>[4x]MAIHNPL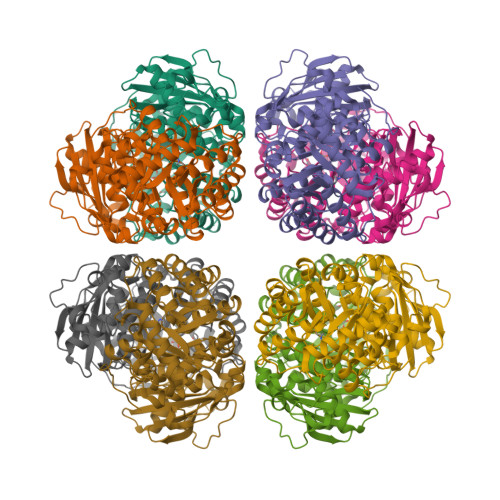AGPKTVKARPTAELSDAYKAGVRAYAVDYYVPDYIPQDTDLLCAFRIQPRGVDMIEAAAAVAAESSTGTWTEVWSNQLTDIDFYKAKVYAITGDIAYIAYPLDLFEENSVVNIMSSIVGNVFGFKAVGALRLEDMRIPLALVKTFPGPRVGIYDERVWSNKWDRPLIGGTVKPKLGLSPKAYSTIIYECLSGGLDTSKDDENMNSQPFSRWRDRFMYAQEAVDRAAAETNEFKGHWHNVTAGSTEESLRRLEYAYELGSRMVMFDFLTAGFAASADIFKRAGELDMIVHCHRAMHAVFTRQANHGIAMRVVAKWLRLTGGDHLHTGTVVGKLEGSWNDTLGIIDILRERYVKANLEHGLYFDQDFGGLKASWPVASGGIHVHHVPDLLKIYGNDAFFLFGGGTHGHPDGSRAGAIANRAAVEAVSAGQTLQQAARSCPELRKSLELWADVKFEVVQ> MKYMITSKGDEKSDLLRLNMIAGFGEYDMEYDDVEPEIVISIGGDGTFLSAFHQYEERLDEIAFIGIHTGHLGFYADWRPAEADKLVKLLAKGEYQKVSYPLLKTTVKYGIGKKEATYLALNESTVKSSGGPFVVDVVINDIHFERFRGDGLCMSTP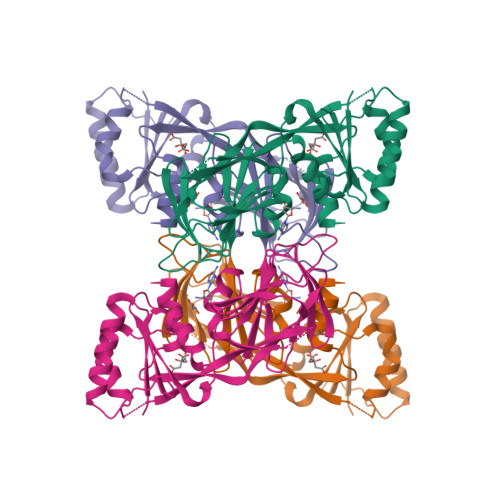SGTTAYNKSLGGALMHPSIEAMQLTEMASINNRVYRTIGSPLVFPKHHVVSLQPVNDKDFQISVDELSILHRDVQEIRYEVSAKKIHFARFRSFPFWRRVHDSFIEDLEHHHHHH6-(4-carboxyphenyl)-3-(4-ethylphenyl)-2~{H}-pyrazolo[3,4-b]pyridine-4-carboxylic acid | C22 H17 N3 O4 | 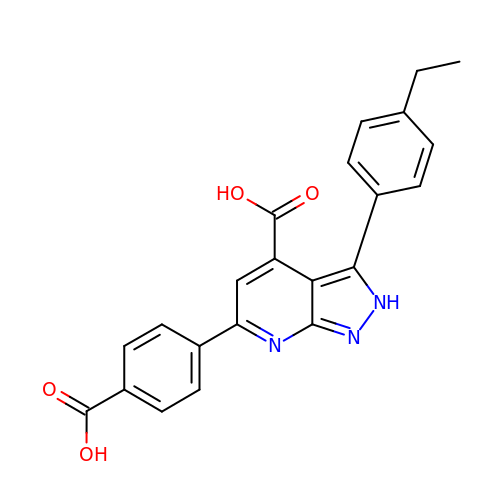AJRMTRZJIPBKHX-UHFFFAOYSA-N(4S)-6-bromo-1,1-dioxido-3,4-dihydro-2H-thiochromen-4-yl 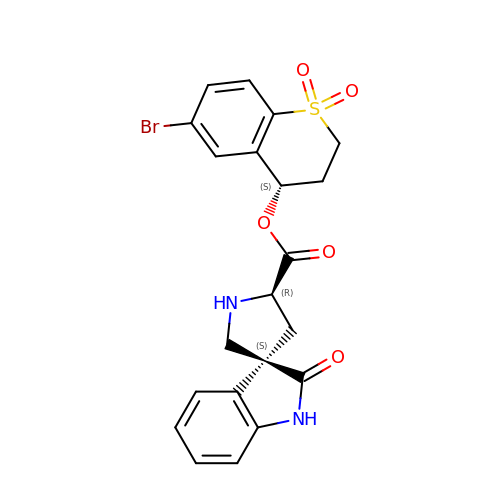(3S,5'R)-2-oxo-1,2-dihydrospiro[indole-3,3'-pyrrolidine]-5'-carboxylate | C21 H19 Br N2 O5 S | AENVIUXFIDGFED-LLGFUMIMSA-N> MVVAGIDPGITHLGLGVVAVEGKGALKARLLHGEVVKTSPQEPAKERVGRIHARVLEVLHRFRPEAVAVEEQFFYRQNELAYKVGWALGAVLVAAFEAGVPVYAYGPMQV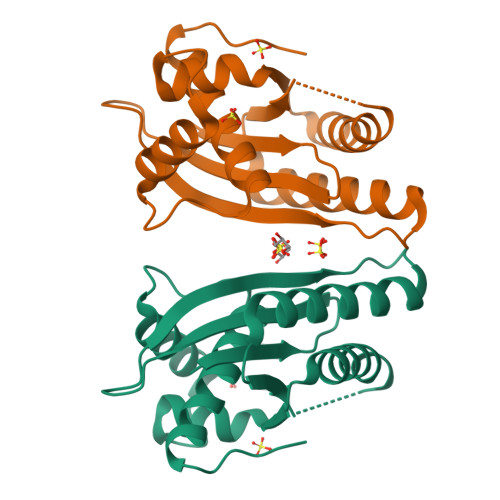KQALAGHGHAAKEEVALMVRGILGLKEAPRPSHLANALAIALTHAFYARMGTAKPL> XXXXXXXXXXXXXXXXXXXXXXXXXXXXXXXXDLRSLERYRADLIDRKILRNKDHGVRAFAACCLSDILRLYAPDAPYTDKELTEIFRLFLAQLKLLQEPENGYLTQQTYLINNLLEYRSIVILTDLPSSSQLVEELFNIFYSPTNSTIQGNMFTAIGGILGEVISECDSLPMSALKMVFNKFLSHKRAESLDGINYKKDPGFEISLIICQTYSNRLGRHFIKFYSEIMYEVLGESDIHEKGIASSAYKTLVKIGNLTSELWKYAPELVGSVTGLLYQLLCSDNELFRESATKCVSKMLGTHSLINFAVAHSDTYKIWLSKMADISPHVR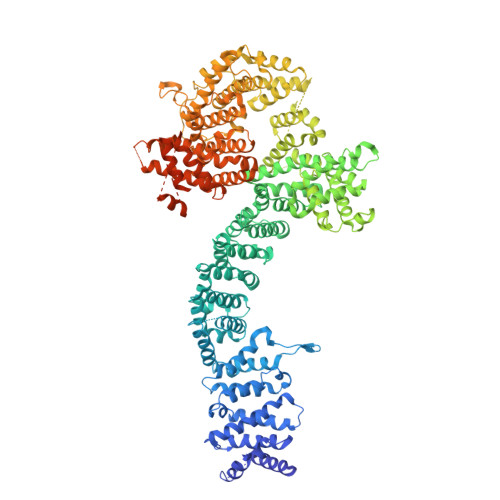QAWVSEIPSILMSRSDLSDDISKGLAKALIDSDHTVRLSAIQTFHEVPVKRLWECLPNAAVFAGLVHLTRETRRDLRDECIDAVARIYTESIESIPKTNENKEIWGVVETIPSACFNLYYINDLEINMKVDLLTFEKFLPLGLSNEEFVQRLLTLLQGFNEKAFSSFYAFNRRQDQMSTVLWKFIEFCEETNSQSPAASLSDTKLIKTVEWISSGFPSHLNVEQILLAFRELNDRRLYRLIKVAVAETSKHLTVRNAVSELFKRLEEPELFRKKNIKIESRFTRDNFSTVFRVLIYRAAPIIFNISNLPSFLNTSDSSNEDEKALKRQLIDNISIIKPGIFKDQVKNLVTIITEGETTGPGNTLSLAEAMRTVYKISKDKREHLDIEENTFFFQKLEDYAKEGNPLEAKYAIKLLGLAPNAAEYLSEVATAILPLDLKSKHFASNVLVLAEITKMQPQLLEKDSTEIVGLLIKDVLLSNDVVGDEDDQQAWFSDEDIYTGKADALSAKVFSLKLFANKIKVMAPDAHADEMTHAFTERTLKLFFYLVASGGELVSESNTDNYPTPANYQNKLRCCAGLHILKITKIASLSRFIKPQDISKLMNLVEDESLEVRSSFIGRLKDFLGDGSISIKFLPLVFFTAYEPDQALRTSTKMWINYTLSKENFRKGTFFERALPRLIHFIAHHPDVAEGLRLRETAFLTGLTTAIDYLVFYADSVLKASNLALLYYLAGRVRQYXXXXXXXXXXXXXXXXXXXXXXXXXXXXXXXXXXXXXXXXXXXXXXXXXXXXXXXXXXXXXXXXXXXXXXXXXXXXXXXXXXXXXXXXXXXXXXXXXXXXXXXXXXXXX> MRNGLVWLLHPALPSTLHSILGARPPPVKRLCGFPKQIYSTMNNPAIQRIEDHIVKSPEDKREYRGLELANGIKVLLISDPTTDKSSAALDVHIGSLSDPPNIPGLSHFCEHMLFLGTKKYPKENEYSQFLSEHAGSSNAFTSGEHTNYYFDVSHEHLEGALDRFAQFFLCPLFDASCKDREVNAVDSEHEKNVMNDAWRLFQLEKATGNPKHPFSKFGTGNKYTLETRPNQEGIDVREELLKFHSTYYSSNLMAICVLGRESLDDLTNLVVKLFSEVENKNVPLPEFPEHPFQEEHLKQLYKIVPIKDIRNLYVTFPIPDLQQYYKSNPGHYLGHLIGHEGPGSLLSELKSKGWVNTLVGGQKEGARGFMFFIINVDLTEEGLLHVEDIILHMFQYIQKLRAEGPQEWVFQECKDLNAVAFRFKDKERPRGYTSKIAGKLHYYPLNGVLTAEYLLEEFRPDLIDMVLDKLRPENVRVAIVSKSFEGKTDRTEQWYGTQYKQEAIPEDVIQKWQNADLNGKFKLPTKNEFIPTNFEILALEKDATPYPALIKDTAMSKLWFKQDDKFFLPKACLNFEFFSPFAYVDPLHCNMAYLYLELLKDSLNEYAYAAELAGLSYDLQNTIYGMYLSVKGYNDKQPILLKKITEKMATFEIDKKRFEIIKEAYMRSLNNFRAEQPHQHAMYYLRLLMTEVAWTKDELKEALDDVTLPRLKAFIPQLLSRLHIEALLHGNITKQAALGVMQMVEDTLIEHAHTKPLLPSQLVRYREVQLPDRGWFVYQRRNEVHNNCGIEIYYQTDMQSTSENMFLELFCQIISEPCFNTLRTKEQ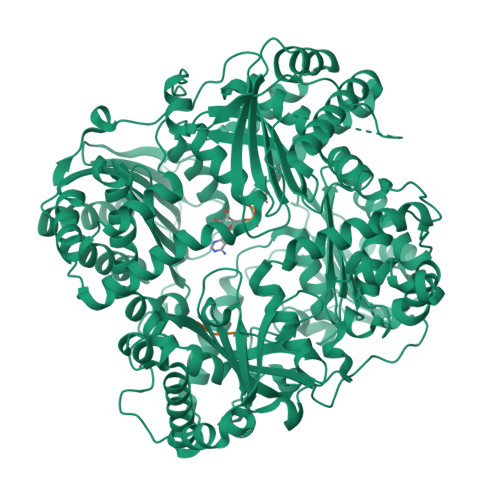LGYIVFSGPRRANGIQGLRFIIQSEKPPHYLESRVEAFLITMEKAIEDMTEEAFQKHIQALAIRRLDKPKKLSAECAKYWGEIISQQYNYDRDNIEVAYLKTLSKDDIIKFYKEMLAVDAPRRHKVSVHVLAREMDSCPVVGEFPSQNDINLSEAPPLPQPEVIHNMTEFKRGLPLFPLVKPHINFMAAKL(3S)-3-AMINO-4-(1H-INDOL-3-YL)BUTANOIC 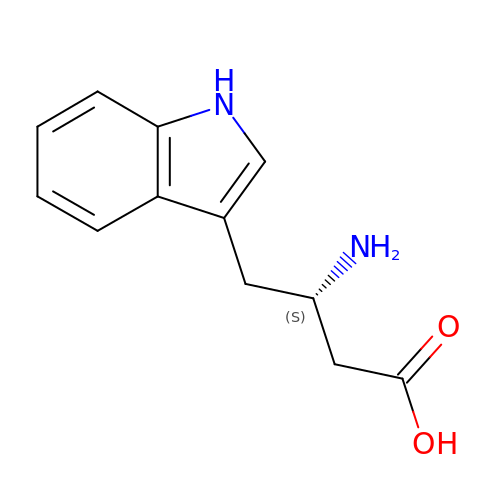ACID | C12 H14 N2 O2 | DUVVFMLAHWNDJD-VIFPVBQESA-N> LNRLREPLLRRLSELLDQAPEGRGWRRLAELAGSRGRLRLSCLDLEQCSLKVLEPEGSPSLCLLKLMGEKGCTVTELSDFLQAMEHTEVLQL;> EEDLTEVKKDALENLRVYLCEKIIAERHFDHLRAKKILSREDTEEISCRTSSRKRAGKLLDYLQENPKGLDTLVESIRREKTQNFLIQKITDEVLKLRNIKLEHLK

CARD11, B cell lymphoma 10 (BCL10) and mucosa-associated lymphoid tissue lymphoma translocation protein 1 (MALT1) assemble the CARD11-BCL10-MALT1 (CBM) complex that bridges TCR/BCR proximal signaling to the canonical IκB kinase (IKK)/NF-κB and JNK pathway in lymphocytes. Upon assembly, the CBM complex serves as a scaffolding platform that activates downstream signaling events via association of mediators such as ubiquitin ligases (e.g., TRAF6) and protein kinases (e.g., TAK1 and IKKβ). Beyond the scaffolding function, MALT1 is a paracaspase and contributes proteolytic activity to the CBM complex, which is key for optimal lymphocyte activation and differentiation. CARD11 acts as a molecular seed that upon binding induces the assembly of BCL10 filaments in vitro and in cells.

To provide structural information about the interaction of BCL10 with MALT1 we performed cryo-electron microscopy (cryo-EM) of the human BCL10 (full length)-MALT1 (T29-G722) complex. Visual inspection of cryo-EM images of the purified complex, underpinned by 2D classification and examination of the power spectra, revealed that BCL10-MALT1 assembles into flexible helical filaments of ~29 nm in diameter, with an ordered inner core of ~14 nm in diameter and a less defined periphery. Our analysis revealed that BCL10-MALT1 is a left-handed helix with a per subunit rotation of 100.8° and a rise of 5.083 Å, resulting in 3.571 subunits of BCL10-MALT1 per helical turn. This helical arrangement agrees with the one observed for the BCL10 (residue 1–115) filament alone, thus indicating that the overall arrangement of the BCL10 CARD core is largely unaltered within the BCL10-MALT1 complex structure. The 4.9 Å resolution map of the inner filament part enabled us to build a pseudo atomic model of BCL10 residues 10–115 and MALT1 residues (30–121) by flexible fitting of a BCL10 homology model and a related crystal structure of MALT1 DD into the EM density. Whereas type I and type II interactions are interstrand contacts between the helical turns, the type III interface exhibits interactions in the helical-strand direction. The MALT1 DD interacts with BCL10 at the rim of the CARD core filament in a 1:1 stoichiometry. A close-up view of the BCL10-MALT1 interaction site I (BM-I) illustrates that MALT1 binds to the C-terminal part (BCL10 helix α6) of the BCL10 CARD forming a new interface that is distinct from the BCL10 filament interfaces I–III. In BM-I, the two most central interacting residues of MALT1 are V81 and L82 situated in helix α4.>MGSSHHHHHHSQDPMIRCLRLKVEGALEQIFTMAGLNIRDLLRDILRRWRDENYLGMVEGAGMFIEEIHPEGFSLYVHLDVRAVSLLEAIVQHLTEAIISSLAVEFDHATGGERVHLIDLHFEVLDNLLE[2x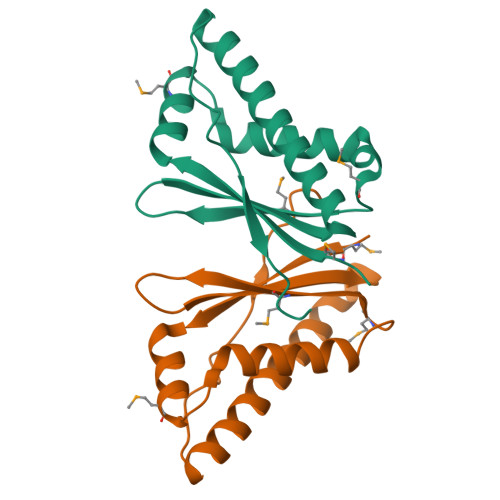]> SSGAIIYTVELKRYGGPLGITISGTEEPFDPIIISSLTKGGLAERTGAIHIGDRILAINSSSLK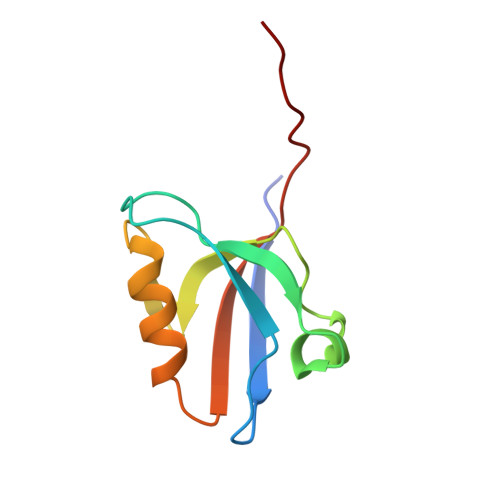GKPLSEAIHLLQMAGETVTLKIKKQTDAQPASS>[2x]GNNVVVLGTQWGDEGKGKIVDLLTERAKYVVRYQGGHNAGHTLVINGEKTVLHLIPSGILRENVTSIIGNGVVLSPAALMKEMKELEDRGIPVRERLLLSEACPLILDYHVALDNAREKARGAKAIGTTGRGIGPAYEDKVARRGLRVGDLFDKETFAEKLKE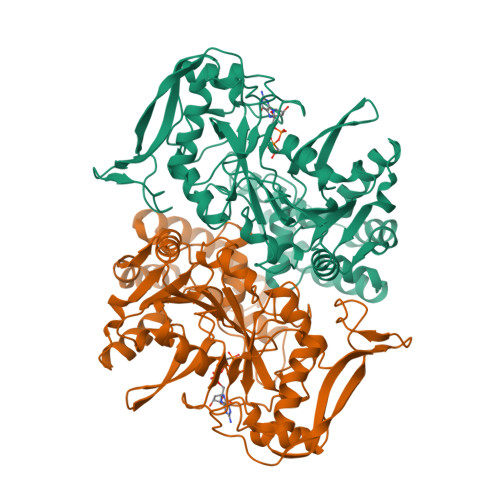VMEYHNFQLVNYYKAEAVDYQKVLDDTMAVADILTSMVVDVSDLLDQARQRGDFVMFEGAQGTLLDIDHGTYPYVTSSNTTAGGVATGSGLGPRYVDYVLGILKAYSTRVGAGPFPTELFDETGEFLCKQGNEFGATTGRRRRTGWLDTVAVRRAVQLNSLSGFCLTKLDVLDGLKEVKLCVAYRMPDGREVTTTPLAADDWKGVEPIYETMPGWSESTFGVKDRSGLPQAALNYIKRIEELTGVPIDIISTGPDRTETMILRDPFDA>MATPWSGYLDDVSAKFDTGVDNLQTQVTEALDKLAAKPSDPALLAAYQSKLSEYNLYRNAQSNTVKVFKDIDAAIIQNFR[19x];>MLNIQNYSASPHPGIVAERPQTPSASEHVETAVVPSTTEHRGTDIISLSQAATKIHQAQQTLQSTPPISEENNDERTLARQQLTSSLNALAKSGVSLSAEQNENLRSAFSAPTSALFSASPMAQPRTTISDAEIWDMVSQNISAIGDSYLGVYENVVAVYTDFYQAFSDILSKMGGWLLPGKDGNTVKLDVTSLKNDLNSLVNKYNQINSNTVLFPAQSGSGVKVATEAEARQWLSELNLPNSCLKSYGSGYVVTVDLTPLQKM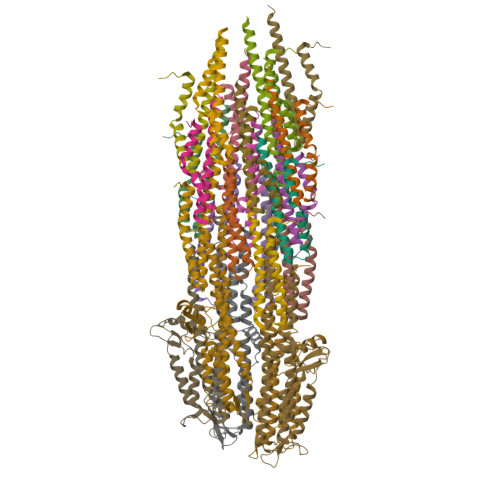VQDIDGLGAPGKDSKLEMDNAKYQAWQSGFKAQEENMKTTLQTLTQKYSNANSLYDNLVKVLSSTISSSLETAKSFLQG[5x]>[4x]MVPISPIETVPVKLKPGMDGPKVKQWPLTEEKIKALVEICTELEKEGKISKIGP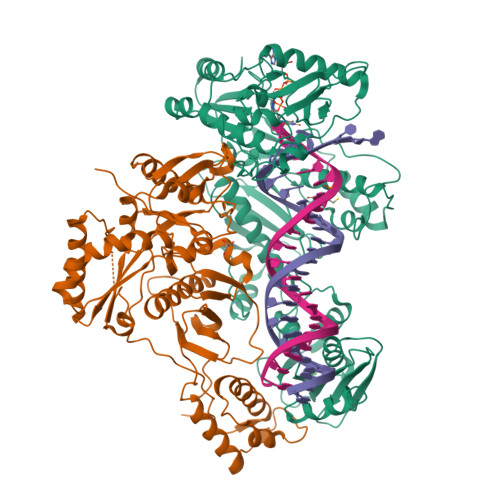ENPYNTPVFAIKKKNSTRWRKLVDFRELNKRTQDFWEVQLGIPHPAGLKKKKSVTVLDVGDAYFSVPLDEDFRKYTAFTIPSINNETPGIRYQYNVLPQGWKGSPAIFQSSMTKILEPFKKQNPDIVIYQYMDDLYVGSDLEIGQHRTKIEELRQHLLRWGLYTPDQKHQKEPPFLWMGYELHPDKWTVQPIVLPEKDSWTVNDICKLVGKLNWASQIYPGIKVRQLSKLLRGTKALTEVIPLTEEAELELAENREILKEPVHGVYYDPSKDLIAEIQKQGQGQWTYQIYQEPFKNLKTGKYARMRGAHTNDVKQLTEAVQKITTESIVIWGKTPKFKLPIQKETWETWWTEYWQATWIPEWEFVNTPPLVKLWYQLEKEPIVGAETFYVDGAANRETKLGKAGYVTNKGRQKVVPLTNTTNQKTELQAIYLALQDSGLEVNIVTDSQYALGIIQAQPDKSESELVNQIIEQLIKKEKVYLAWVPAHKGIGGNEQVDKLVSAGIRKVL;>PISPIETVPVKLKPGMDGPKVKQWPLTEEKIKALVEICTEMEKEGKISKIGPENPYNTPVFAIKKKDSTKWRKLVDFRELNKRTQDFWEVQLGIPHPAGLKKKKSVTVLDVGDAYFSVPLDEDFRKYTAFTIPSINNETPGIRYQYNVLPQGWKGSPAIFQSSMTKILEPFKKQNPDIVIYQYMDDLYVGSDLEIGQHRTKIEELRQHLLRWGLTTPDKKHQKEPPFLWMGYELHPDKWTVQPIVLPEKDSWTVNDIQKLVGKLNWASQIYPGIKVRQLSKLLRGTKALTEVIPLTEEAELELAENREILKEPVHGVYYDPSKDLIAEIQKQGQGQWTYQIYQEPFKNLKTGKYARMRGAHTNDVKQLTEAVQKITTESIVIWGKTPKFKLPIQKETWETWWTEYWQATWIPEWEFVNTPPLVKLWYQGGHHHHHHH[4x]>[8x]MSEKYIVTWDMLQIHARKLASRLMPSEQWKGIIAVSRGGLVPGALLARELGIRHVDTVCISSYDHDNQRELKVLKRAEGDGEGFIVIDDLVDTGGTAVAIREMYPKAHFV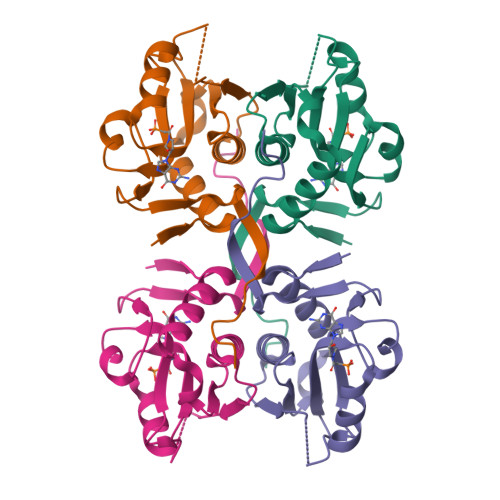TIFAKPAGRPLVDDYVVDIPQDTWIEQPWDMGVVFVPPISGR>[2x]EAEAEFGACGAIASTVPNYNNAKLPDPFTFANGTALRTKADWSCRRAEISALIQNYEAGTLPPKPPVVTASFSKSGNTGTLAITAGLSNSQTIKFSPTISYPSGTPPANGWPLIIAYEGGSIPIPAGVATLTYSNSDMAQQNSASSRGQGLFYQLYGSTHSASAMTAWVWGVSRIIDALEMTPTAQINTQRIGVTGCARDGKGALMAGAFEERIALTIPQESGSGGDACWRLSKYEIDNGNQVQDAVEIVGENVWFSTNFNNYVQKLPTVPEDHHLLAAMVAPRAMISFENTDYLWLSPMSSFGCMTAAHTVWQGLGIADSHGFAQVGGHAHCAWPSSLTPQLNAFINRFLLDQSATTNVFTTNNQFGKVQWNAANWITWTTPTLTENLYFQGVDHHHHHH

A common type of LCC in hardwood is the ester-LCC formed between α-1,2-linked 4-O-methyl-d-glucuronoyl moieties of acetylated glucuronoxylan and γ-alcohols in lignin. It was recently discovered that an insoluble hardwood lignin-preparation (LRP) is amenable to enzymatic hydrolysis by a glucuronoyl esterase (GE, EC 3.1.1.B11) releasing aldouronic acids. WT CuGE has a modular architecture with a N-terminal carbohydrate-binding module 1 (CBM1) domain connected to the catalytic domain by a proline-rich linker region. The overall fold of the catalytic domain of CuGE features a large ten-stranded twisted β-sheet flanked by α-helical elements and a surface-exposed active site. The structure complies with the characteristics of a serine esterase belonging to the α/β-hydrolase superfamily.

The aldouronic acid ligands dock onto the surface of CuGE in all the complexes: dΔS270A:Um4X, dΔS270A:Um4XX-OH and dΔS270A:XUm4XX-OH without any major conformational changes of the slightly twisted, branched oligosaccharide. Structures of ligand-bound complexes showed that the ligands bind in the highly accessible and solvent exposed binding site of molecule B only. The α-1,2-linked 4-O-methyl-d-glucuronoyl moiety is nested in the small substrate-binding pocket, that provides distinct recognition of all hydroxyl groups and a hydrophobic environment for accommodation of the 4-O-methyl-d-glucuronoyl substituent, while the xylan-backbone runs along the surface and displays only hydrophobic, van der Waals and water-mediated interactions with the protein. All hydroxyl groups in the 4-O-methyl-d-glucuronoyl moiety are engaged in hydrogen bonds and the free carboxylate group displays polar interactions with both the catalytic H404 and R271. We observe that binding of aldouronic acids is coupled to a conformational change of R271 that allows the side chain to engage in substrate recognition and complete the formation of the oxyanion hole. Thus, the oxyanion hole is created solely by R271 with both the backbone amide and guanidinium side chain nitrogen atoms forming close contacts with the O6 carbonyl of the 4-O-methyl-glucuronoyl moiety (3.2 and 2.8 Å, respectively), mimicking the interactions in a tetrahedral reaction intermediate. In the complex formed at pH 7.5–8 (dΔS270A:U4mX), Y366 moves “out” upon substrate binding, and no significant differences are observed in substrate recognition interactions compared to the complexes formed at pH 5.5 (dΔS270A:Um4XX-OH and dΔS270A:XUm4XX-OH). MST measurements of ΔWT and dΔS270A respectively on aldotetrauronic acid (Um4XX-OH) indicate equilibrium dissociation constants in the mM range with a moderately stronger binding (one order of magnitude) between dΔS270A and Um4XX-OH compared to the active variant. The strong binding in dΔS270A:Um4XX-OH is in accordance with the well-defined binding observed in the complexes of CuGE.>RYNDYKLDFRRQQMQDFFLAHKDEEWFRSKYHPDEVGKRRQEARGALQNRLRVFLSLMETGWFDNLLLDIDKADAIVKMLDAAVIKMEGGTENDLRILEQ[2x];>GLECKPRPLHKTCSLFMRNIAPNISRAEIISLCKRYPGFMRVALSEPQPERRFFRRGWVTFDRSVNIKEICWNLQNIRLRECELSPGVNRDLTRRVRNINGITQHKQIVRNDIKLAAKLIHTLDDRTQLWASEPGTPPLPTSLPSQNPILKNITDYLIEEVSAEEEELLGSSGGAPPEEPPKEGNPAEINVERDEKLIKVLDKLLLYLRIVHSLDYYNTCEYPNEDEMPNRCGIIHVRGPMPPNRISHGEVLEWQKTFEEKLTPLLSVRESLSEEEAQKMGRKDPEQEVEKFVTSNTQELGKDKWLCPLSGKKFKGPE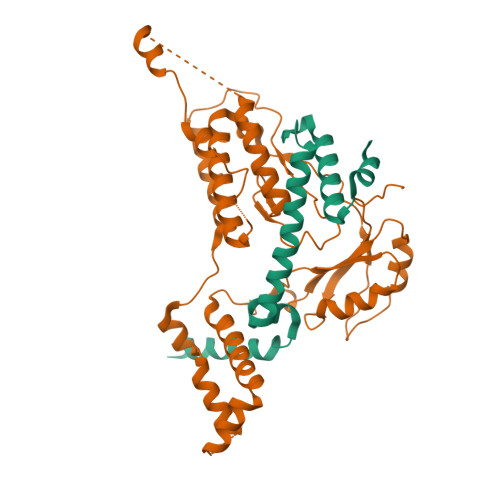FVRKHIFNKHAEKIEEVKKEVAFFNNFLTDAKRPALPE[2x]> KPRIDMHSHFFPRISEQEAAKFDANHAPWLQVSAKGDTGSIMMGKNNFAPVYQALWDPAFRIEEMDAQGVDVQVTCATPVMFGYTWEANKAAQWAERMNDFALEFAAHNPQRIKVLAQVPLQDLDLACKEASRAVAAGHLGIQIGNHLGDKDLDDATLEAFLTHCANEDIPILVHPWDMMGGQRMKKWMLPWLVAMPAETQLAILSLILSGAFERIPKSLKICFGHGGGSFAFLLGRVD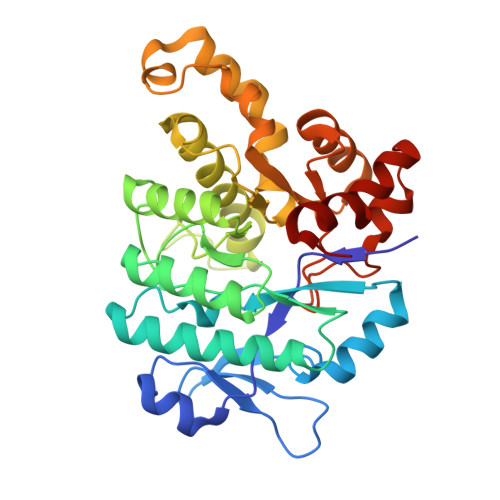NAWRHRDIVREDCPRPPSEYVDRFFVDSAVFNPGALELLVSVMGEDRVMLGSDYPFPLGEQKIGGLVLSSNLGESAKDKIISGNASKFFNIN>GAMSTTSTTIQVIGAGLPRTGTNSMKKALEIIYSKPCYHMYEIIFKKQSDISIWQQLIDETHKTTSD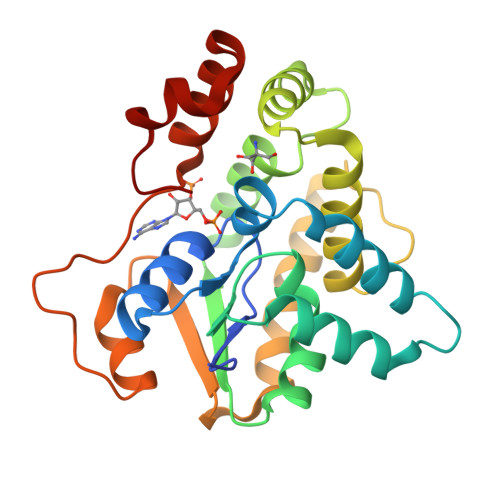KRKIYNGLNELLNGYIATTDLPSCSFYKELMTMYPNAKVLLTIRDKYDWLYSLRKVVLPKSTDPWKLKIEEGDQVLGIDSNFYKMTEDSLKFAFQKNHINLDDDEILLECYDEYNRLVQEIVPPERLLIHHLGDGWESLCQFLNVDIPNGISYPCANSHHQMTQLTEQLIKHKSLDDIIHMFPGLI[2x]>ESEHTEVSLALFNYDDINVKVDFILLEKNMTINELKMYVENELFKFPDDIVKHVNIKVNGSLVGHGELVSIEDGYGIEISSWMVKE[4x]

Non‐flagellar type III secretion systems (NF‐T3SS) are essential for initiating infection by many pathogenic Gram‐negative bacteria. In particular, the protein Spa33 (SctQ), which is essential for secretion and localises to the base of the S. flexneri NF‐T3SS in situ via association with the basal body (Morita‐Ishihara et al., 2006; Barison et al., 2012), has been proposed to form a substructure termed the cytoplasmic‐ring (C‐ring) (Morita‐Ishihara et al., 2006). In this study, we show that alternative translation occurs to generate full‐length Spa33 (Spa33‐FL) and a shorter C‐terminal fragment (Spa33‐C) within S. flexneri, with the production of both being required for assembly and function of the NF‐T3SS. High resolution biophysical studies demonstrate that Spa33‐FL and Spa33‐C associate to form a minimal 1:2 complex that then undergoes further oligomerisation to produce elongated arrays.

The 2.3 Å resolution crystal structure of Spa33208‐293 was subsequently determined by molecular replacement. The structure shows a SpoA domain that forms the expected saddle‐shaped homodimer with an approximate twofold rotational symmetry axis. Regions of notable asymmetry have high B‐factors, suggesting conformational flexibility accounts for major differences between the dimer halves. Indeed superimposition of Spa33208‐293 with T. maritima FliN (Brown et al., 2005) (2.18 Å RMSD, 126 Cα atoms), Yersinia pseudotuberculosis YscQ‐C (Bzymek et al., 2012) (2.09 Å RMSD, 135 Cα atoms) and Pseudomonas syringae HrcQB‐C (Fadouloglou et al., 2004) (2.40 Å RMSD, 133 Cα atoms) shows a remarkably similar arrangement of secondary structure elements. In order to gain insights into the interaction of Spa33‐FL with Spa33‐C2, the intermolecular contacts of the Spa33208‐293 crystal were investigated and revealed a dimer–dimer interface formed by an equivalent surface of each homodimer, comprising regions proximal to the N‐terminus, C‐terminus and β3‐β4 turn from one chain and α1 from the other. This interaction buries a surface area of 508 Å2 and is stabilised by three hydrogen bonds and hydrophobic interactions between apolar residues that are conserved with SpoA1 of Spa33‐FL and orthologous domains. In particular, Tyr221 makes a significant contribution to the interaction, fitting into a hydrophobic pocket formed by the interacting dimer (Val265/Val270/Trp289/Val291 and Ile239/Leu242/Lys243 of opposing chains). In contrast to the closed tetramer of FliN, the Spa33208‐293 and HrcQB‐C assemblies form an open lock washer structure, with the concave surfaces of the saddle‐shaped dimers being offset laterally by ∼ 55° with respect to each other. Indeed, a continuous spiral of Spa33208‐293 dimers is observed in the crystal lattice, providing a molecular model for formation of higher molecular weight oligomers by the analogous dimers of Spa33‐FL/C2.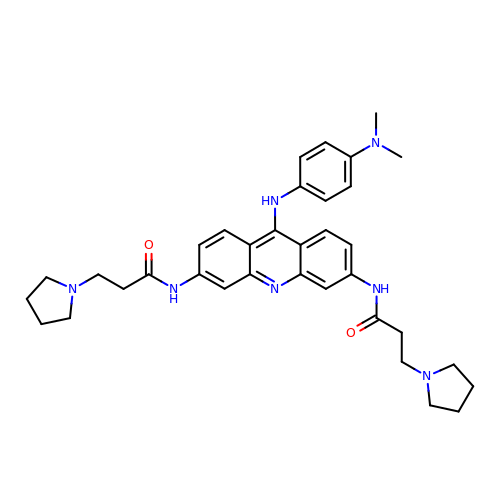9-[4-(n,n-dimethylamino)phenylamino]-3,6-bis(3-pyrrolidinopropionamido) acridine | C35 H43 N7 O2 | RKPYSYRMIXRZJT-UHFFFAOYSA-N>MTPEECRAQYRLMLKEAMDAYHQLNLGGSVRVVVDQNSERVEYTAANRQSLWAYIVRLQNAINSDNPCAAFMGLPSSPAGFLFP[2x];> MSQRLDILKALTAHLEQITIANGYAYDLKGKVYRGRDRFGADFTSRLPIVSILEAKATDYGSFANEEQTVRMDDWVLLVQGWVKDDPRNPTDPAYELLAEVEKRLAMLVAKDEQGQPMYPALYRLGGKIAKLTLAQPVVRPPEDGLSDTAFFFLPVRVGLKVDIRNP;>MTEKKRSTTQRAKKAAKTADVATLDATPQNPSALGGGLEGAERNTREMFRWTPAIISPDQQIAQDGTLALSRAQDIVQNDGYAFGAVAIHRDSVVGSQYKLNSKPNSLVLGAPEGWAEEFQEVVEARFNMVAESPENWFDARRMNTLTGLVRLAVGGFIMTGEVLASCEWMKPNGTRMQRRPFGTAIQMISPYRLSNPDNIMDDKYLRSGVKLDEMGAPIGYWLRKAFPGDPTDLEQWRWEYQPARFDWGRRRMIHIIEALLPGQTRGISEMVAALKQMKMTRNFQEVTLQNAIVNATYAAAIESELPSDVVFNQMGMGQTPFGDILKTYMGSLAEYIAGSKNIAIDGAKIPHLFPGTKLKMQPAGTPGGVGTDYEESLLRNIAASLGLSYEQFSRDYTKTNYSSARASMAETWKYMESRKKLVADRFASMIYTLWLEEEVNAGNVPLPPGFTWRDFYDPMKRDALCNAEWIGASRGQIDEKKETEAAILRIKNGLSTYEAEIARLGGDFREVFKQRAREEGIIKDLGLDFSGKMVEGTEASGSTGSTGSDNNNEEDTKE[2x];> MASNFAAIKAKARRDVHASLSVPARYENYSQDVIVEDLSVRWHNKIAIMGDLENGGYANIVEGIERIIFTREELAVKGVVLSEGDSIIMTAEGYENARLVLKTQEPIVGPVEVVWQVARAD;>MNDNYQNNYVVGRGTVYFDRFQDGTNRKTGEMYFGNTPEFTINTDSETLDHYSSDHGMRVMDASVLLEASQGGTFTCDNINADNLALWFLGEVSNTTQTQQTDAKEVFNPIMRGRYYQLGTTDDNP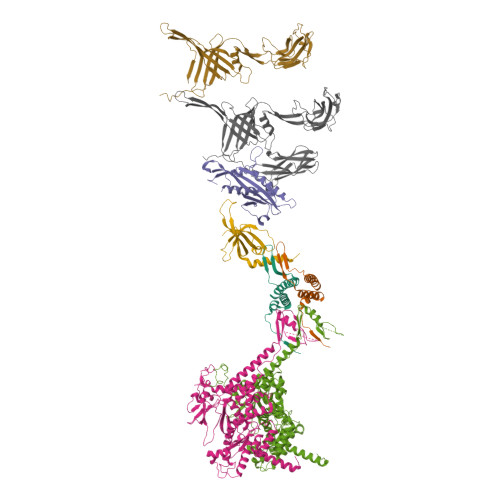TGVRGVTNFQMVKADASIAISVGSGDITSIVGATVVNPAGNYEIDLEAGRIYIEPDSTDLSGNVQIAVQYDVDAQKRTLVIGKSNMVYGALRMISDNPVGLNKNYYFPKVSIAPDGDYALKGDDWQVMSFTFKAMQLNNITQRVYIDIVEAAAAVDPTAQRTIEITPASTTATTGGAGVVCTVTVRDGTGTAVQGDAVTFTTVAGATVTPNSATTGATGTATTTVNRAAAGTATVTATLANGKAATTGTITFSAP[2x]Endo-galactosaminidases are an underexplored family of enzymes involved in the degradation of galactosaminogalactan (GAG) and other galactosamine-containing cationic exopolysaccharides produced by fungi and bacteria. Whereas the fungal enzyme belongs to family GH114, the two bacterial enzymes do not lie in the current GH families but instead define a new family, GH191. The TIM-barrel core structure with fully conserved active-site residues and a negatively charged substrate crevice is conserved among all the families. The putative active-site residues (Asp156/Glu225 for TmGH191, Asp323/Glu391 for Env-GH191 and Asp157/Glu225 for FsGH114) overlap well with the experimentally verified nucleophile and general acid/base Asp189/Glu247 in Ega3, Asp196/Glu222 in Sph3 and Asp160/Glu223 in PelAH.

Here, we describe structure–function investigations of two bacterial enzymes: an enzyme from Thermotoga maritima previously suggested to be a galactosaminidase and another from an environmental sample (termed Env-GH191 here), which has 99.2% identity to an enzyme from Myxococcus fulvus with NCBI reference WP_074950922.1. We could not detect any binding, or enzymatic cleavage of the GAG oligomers, for the T. maritima enzyme, which raises the question as to whether the T. maritima enzyme is an endo-galactosaminidase or whether GAG is not a substrate for this family. The enzyme from the environmental sample was tested with purified Pel and showed good activity towards the isolated Pel, with a preference for GalN-rich oligosaccharides, confirming that the new family GH191 has members with galactosaminidase activity, with a preference for partially deacetylated stretches of Pel. While the GH135 and GH166 families are both retaining α-N-acetyl­galactos­aminidases, GH166 enzymes also have a preference for partially deacetylated stretches compared with the GH135 enzymes, which is in line with the observed specificity of Env-GH191. The two GH191 enzymes overlap well on each other, with an r.m.s.d. of 1.48 Å over 252 residues, while only having a sequence identity of 28%. Whereas helices α1, α6 and α8 are absent in Ega3, both bacterial GH191s contain the α1 helix as a structural element. A comparison of the substrate-binding crevices shows that beyond subsite −3 in both bacterial structures a loop around Asp64 (TmGH191 notation), connecting β2 to α2, partially closes the crevice. To gain better insight into the substrate interactions, we docked the substrate into Env-GH191 and FsGH114. In both cases up to seven subsites could be identified. Whereas the Env-GH191 binding crevice seem to better fit the galactosamine oligomer, the FsGH114 crevice can accommodate either an acetylated or a non-acetylated GAG oligomer equally well. The crystal pathology of Env-GH191 was dealt with using a nonconventional procedure described in Section 2.

>[2x]DAGTPTDAGTPTDAGTPTDAGTPTDAGTQVPWSNVKSFTYQLTNYPQGKLDAIAASKFDLAIVELVRDGSSGYFTAAEISALKARGKQVLAYFEIGAIEEYRPEWSQVPADLKLGPVSGWPDEQYVKYWDERWWPIVQGRIDRALAAGFNGCYLDMVVTYEEIPANSAGTNRADLARKMVALIARINTYAKARNPDFKVVPQNSPELVDDPAYLPAIDGLGMEDMYWSDDVACDEGWCEENRTNAARVRAAGKLVLSTDYATQSAHVADAYTRSRAAGFVPYVTVRALDRVTVNAGWDPQ> MKLYNLKDHNEQVSFAQAVTQGLGKNQGLFFPHDLPEFSLTEIDEML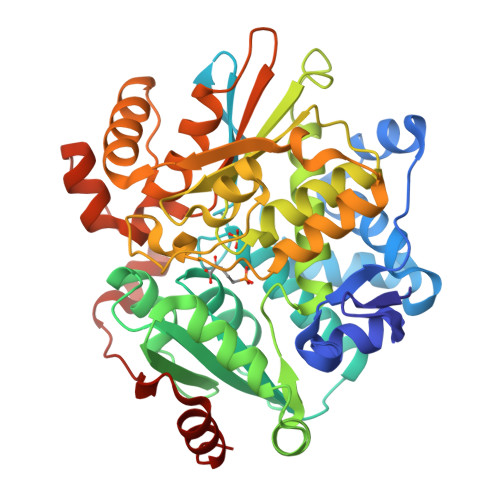KLDFVTRSAKILSAFIGDEIPQEILEERVRAAFAFPAPVANVESDVGCLELFHGPTLAFKDFGGRFMAQMLTHIAGDKPVTILTATSGDTGAAVAHAFYGLPNVKVVILYPRGKISPLQEKLFCTLGGNIETVAIDGDFDACQALVKQAFDDEELKVALGLNSANSINISRLLAQICYYFEAVAQLPQETRNQLVVSVPSGNFGDLTAGLLAKSLGLPVKRFIAATNVNDTVPRFLHDGQWSPKATQATLSNAMDVSQPNNWPRVEELFRRKIWQLKELGYAAVDDETTQQTMRELKELGYTSEPHAAVAYRALRDQLNPGEYGLFLGTAHPAKFKESVEAILGETLDLPKELAERADLPLLSHNLPADFAALRKLMMNHQ>[2x]MSEAAHVLITGAAGQIGYILSHWIASGELYGDRQVYLHLLDIPPAMNRLTALTMELEDCAFPHLAGFVATTDPKAAFKDIDCAFLVASMPLKPGQVRADLISSNSVIFKNTGEYLSKWAKPSVKVLVIGNPDNTNCEIAMLHAKNLKPENFSSLSMLDQNRAYYEVASKLGVDVKDVHDIIVWGNHGESMVADLTQATFTKEGKTQKVVDVLDHDYVFDTFFKKIGHRAWDILEHRGFTSAASPTKAAI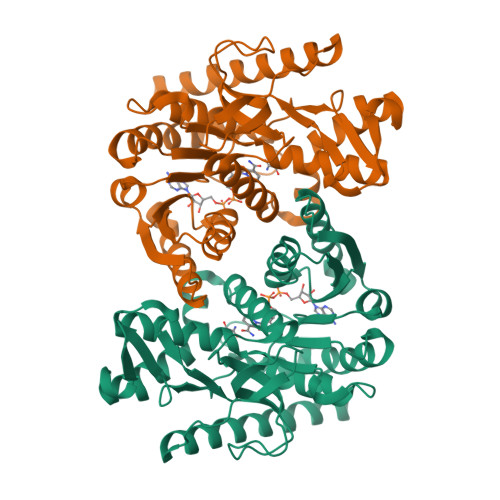QHMKAWLFGTAPGEVLSMGIPVPEGNPYGIKPGVVFSFPCNVDKEGKIHVVEGFKVNDWLREKLDFTEKDLFHEKEIALNHLAQLEHHHHHH>MVQELSIERLLEMESLVADPSEEFQFLRVGPDSNVPP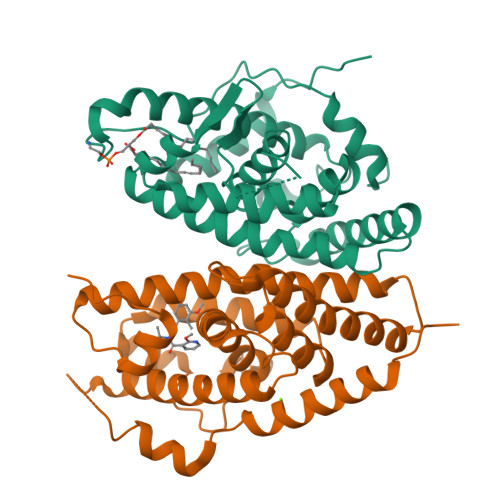KFRAPVSSLCQIGNKQIAALVVWARDIPHFSQLEMEDQILLIKGSWNELLLFAIAWRSMEFLTEERDGVDGTGNRTTSPPQLMCLMPGMTLHRNSALQAGVGQIFDRVLSELSLKMRTLRVDQAEYVALKAIILLNPDVKGLKNRQEVEVLREKMFLCLDEYCRRSRSSEEGRFAALLLRLPALRSISLKSFEHLFFFHLVADTSIAGYIRDALRNHAPPIDTNMM[3x];>[3x]GSHMASMTGGQQMGRDPLKNVPPLTANQKSLIARLVYYQEGYEQPSEEDLKRVTQTWQSDEDDEDSDMPFRQITEMTILTVQLIVEFAKGLPGFSKISQSDQITLLKACSSEVMMLRVARRYDAATDSVLFANNQAYTRDNYRKAGMAYVIEDLLHFCRCMYSMMMDNVHYALLTAIVIFSDRPGLEQPSLVEEIQRYYLNTLRVYILNQNSASPRSAVIFGKILGILTEIRTLGMQNSNMCISLKLKNRKLPPFLEEIWDVADVA>LPVEKIIREAKKILDELLKRGLIDPELARIAREVLERARKLGNE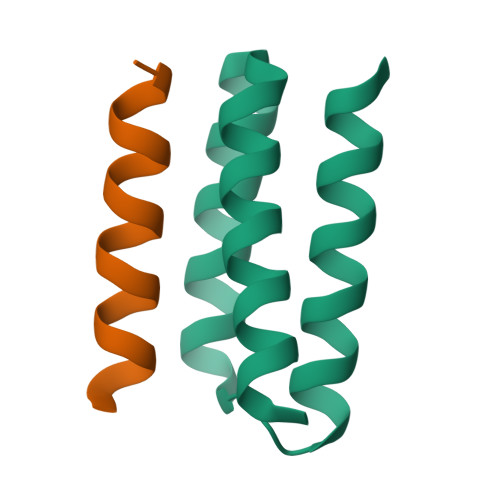EAARFVLELIERLRRELS[2x];>[2x]DEHELLETAARWFYEIAKR>SYATKIHARYVYDSRGNPTVEVDFTTDKGLFRSIVPSGASTGVHEALELRDGDKSKWLGKGVLKAVANVNDIIAPALIKAKIDVVDQAKIDEFLLSLDGTPNKSKLGANAILGVSLAAANAAAAAQGIPLYKHIANISNAKKGKFVLPVPFQNVLNGGSHAGGALAFQEFMIAPTGVSTFSEALRIGSEVYHNLKSLTKKKYGQSAGNVGDEGGVAPDIKTPKEALDLIMDAIDKAGYKGKVGIAMDVASSEFYKDGKYDLDFKNPESDPSKWLSGPQLADLYEQLISEYPIVSIEDPFAEDDWDAWVHFFERVGDKIQIVGDDLTVTNPTRIKTAIEKKAANALLLKVNQIGTLTESIQAANDSYAAGWGVMVSHRSGETEDTFIADLSVGLRSGQ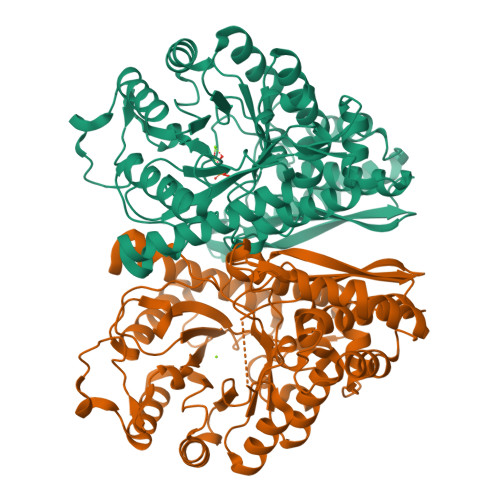IKTGAPARSERLAKLNQILRIEEELGSEAIYAGKDFQKASQL[4x]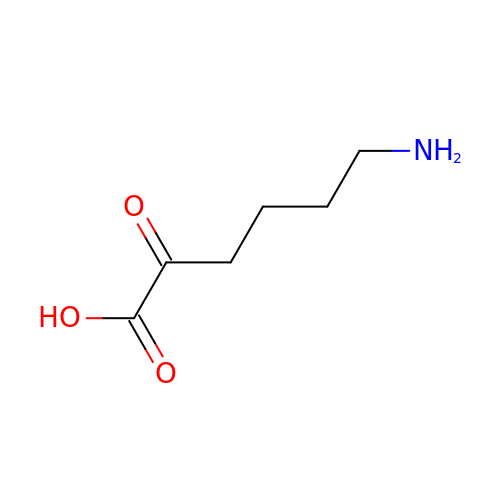6-azanyl-2-oxidanylidene-hexanoic acid | C6 H11 N O3 | GWENQMVPLJAMAE-UHFFFAOYSA-N CTNNBL1 is a spliceosome-associated protein that binds nuclear localization signals (NLSs) in splice factors CDC5L and Prp31 as well as the antibody diversifying enzyme AID. CTNNBL1 is a widely expressed, highly conserved 62 kDa nuclear protein that associates with components of the RNA splicing machinery. CTNNBL1 comprises a HEAT-like domain (including a nuclear export signal), a central armadillo domain, and a coiled-coil C-terminal domain. Our results identify CTNNBL1 as a unique selective NLS-binding protein with striking differences from karyopherin-αs.

We crystallized full-length human 6xHis-CTNNBL1 and N-terminally truncated 6xHis-CTNNBL1Δ76 (to generate a fragment that is necessary and sufficient for NLS-peptide binding). We were unable to solve the structure using molecular replacement and therefore crystallized selenomethionine-substituted protein for experimental phase determination, solving the structures of CTNNBL1Δ76 and that of full-length CTNNBL1 from crystals with the symmetry of different spacegroups. The overall structure of CTNNBL1Δ76 reveals a superhelical coiled coil composed of α-helices stacked against each other to form an extended configuration, in agreement with circular dichroism data. The structure can be divided into three distinct regions: an N-terminal pre-armadillo (PRE-ARM) domain (residues 76–176); a central compact armadillo (ARM) domain with helices tightly packed against one another to form a solenoid (residues 177–416); and a C-terminal domain (CTD) that projects out from the smooth solenoid of the ARM domain (residues 417–562). Residues along the central spine of the solenoid and the CTD have low temperature factors, consistent with their role in stabilizing the core of the molecule, whilst N and C-terminal regions beyond the CTD display higher B-factors for solvent-exposed residues, implying greater flexibility. Preceding the ARM domain is a region (PRE-ARM domain) comprising 6 α-helices and connecting loops, which do not form the ordered triple helical arrays that constitute armadillo repeats. As in HEAT repeats, the CTNNBL1Δ76 PRE-ARM helices also contain conserved hydrophobic residues in the buried interaction surface of the helices where they mediate intra- and inter-repeat packing. In order to probe the NLS binding mode of CTNNBL1, we generated multiple mutants of CTNNBL1Δ76 based on the crystal structure. Strikingly, all mutants retained the ability to interact with the CDC5L NLS3 as judged by a pulldown assay. Thus, CTNNBL1 likely recognizes NLS ligands in a manner very different from karyopherin-α.

> MAHHHHHHMLDESSVKKMILTFEKRSYKNQELRIKFPDNPEKFMESELDLNDIIQEMHVVATMPDLYHLLVELNAVQSLLGLLGHDNTDVSIAVVDLLQELTDIDTLHESEEGAEVLIDALVDGQVVALLVQNLERLDESVKEEADGVHNTLAIVENMAEFRPEMCTEGAQQGLLQWLLKRLKAKMPFDANKLYCSEVLAILLQDNDENRELLGELDGIDVLLQQLSVFKRHNPSTAEEQEMMENLFDSLCSCLMLSSNRERFLKGEGLQLMNLMLREKKISRSSALKVLDHAMIGPEGTDNCHKFVDILGLRTIFPLFMKSPRKIKKVGTTEKEHEEHVCSILASLLRNLRGQQRTRLLNKFTENDSEKVDRLMELHFKYLGAMQVADKKIEGEKHDMVRRGEIIDNDTEEEFYLRRLDAGLFVLQHICYIMAEICNANVPQIRQRVHQILNMRGSSIKIVRHIIKEYAENIGDGRSPEFRENEQKRILGLLENF>[2x]MNVLSVSSEIYPLIKTGGLADVVGALPIALEAHGVRTRTLIPGYPAVKAAVTDPVKCFEFTDLLGEKADLLEVQHERLDLLILDAPAYYERSGGPYLGQTGKDYPDNWKRFAALSLAAARIGAGVLPGWRPDMVHAHDWQAAMTPVYMRYAETPEIPSLLTIHNIA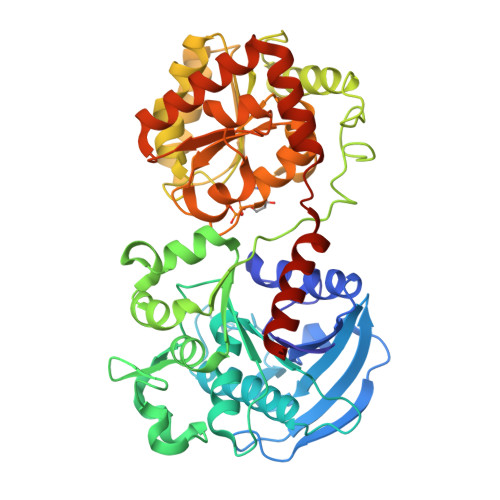FQGQFGANIFSKLALPAHAFGMEGIEYYNDVSFLKGGLQTATALSTVSPSYAEEILTAEFGMGLEGVIGSRAHVLHGIVNGIDADVWNPATDHLIHDNYSAANLKNRALNKKAVAEHFRIDDDGSPLFCVISRLTWQKGIDLMAEAVDEIVSLGGRLVVLGAGDVALEGALLAAASRHHGRVGVAIGYNEPLSHLMQAGCDAIIIPSRFEPCGLTQLYALRYGCIPVVARTGGLADTVIDANHAALASKAATGVQFSPVTLDGLKQAIRRTVRYYHDPKLWTQMQKLGMKSDVSWEKSAGLYAALYSQLISKGHHHHHH>[2x]GPSGGGADVNKGPWAMALTPMEFARKYNLLRKDDALLDNPVPGEEMTAGIRRGDAKRVFTMQLGPYWDGFERCSPQAYALSAVFMARMNRDRDAANNILKVLDKTFVDGKPDFSVARPVMKKYQNSELVQEVVAKHAYVLTVIASLLEAAREDGVVPSSEFLWLKPVDRRLWYMLNCVGRQTPYSEVAGPFAHWKAEKEMGRRSLVPMIDEAIRALEIAVKEVRLTPRQMEELEP

The T4BS secretion coupling complex of L. pneumophila comprises the inner membrane AAA+ ATPase DotL (IcmO) and two inner membrane/cytoplasmic components, DotM (IcmP) and DotN (IcmJ). In this study, we determine the crystal structure of the cytoplasmic domain of DotM and observe large patches of basic residues, leading us to hypothesize that DotM might form the recruiting platform for Glu-rich motif-containing effectors. Our results suggest that DotM’s cytoplasmic domain is capable of binding directly another subgroup of Legionella effectors that contain acidic Glu-rich motifs at their C terminus.

Thus, a shorter construct (residues 153–380, referred thereafter as DotM153) was cloned, expressed, and purified. DotM153 crystals however diffracted to 1.8 Å resolution. These crystals contained two molecules in the asymmetric unit. The DotM153 crystal structure is similar to that published by Kwak et al. (PDB entry code 5 × 1U; root mean square deviation (RMSD) in Cα atoms of 0.4 Å) and reveals an all-α-helical fold, comprising 13 α-helices connected by loops, many of them proline-rich. Residues 179–188 in monomer A in the loop connecting helices α1 and α2 were not resolved, indicating flexibility in this region of the protein. The pear-shape structure is formed of a narrower end made by two elongated sequences emanating from both the N- and C-terminal regions of the sequence: α1, α2, and part of the α3 on one side and α13 and α12 on the other. The remaining α-helices (α4 to α11) form a larger compact structure with helices α7, α8, α9, and α10 tightly wrapping around a helical bundle formed by α4, α5, and α6. While the structural homology search and structure-based sequence alignment yielded no clue as to the function of DotM, functional implications could however be derived from a striking feature of the DotM153 structure: its highly charged surface. Indeed, DotM153 contains 33 surface-exposed Lys/Arg and 28 surface-exposed Glu/Asp residues scattered around the entire surface of the protein. Peptides CegC3, Lpg1663, and OSM that contain a Glu-rich motif exhibited high affinity to DotM153 (KD values of 0.19, 0.7, and 0.35 μM, respectively), whereas Lem21 and LegC8 which do not contain C-terminal Glu-rich motifs did not bind.> MSKLNAYFGEYGGQFVPQILVPALDQLEQEFIKAQADESFKQEFKELLQEYAGRPTALTKTRNIVKNTRTKLYLKREDLLHGGAHKTNQVLGQALLAKRMGKKEIIAETGAGQHGVATALACALLDLKCRVYMGAKDVERQSPNVFRMKLMGAEVIPVHSGSATLKDACNEALRDWSANYSKAHYLLGTAAGPHPFPTIVREFQRMIGEETKQQMLAKEGRLPDAVIACVGGGSNAIGMFADFIDEKNVKLIGVEPAGKGIETGEHGAPLKHGKTGIFFGMKAPLMQNSDGQIEESYSISAGLDFPSVGPQHAHLLAIGRAKYASAT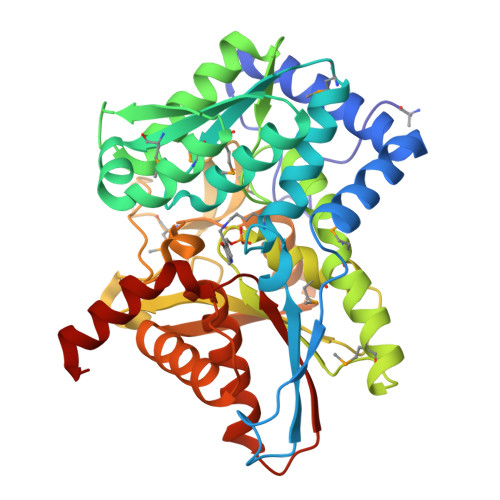DDEALDAFKLLCKKEGIIPALESSHALAHALKLAYEDPNKEQLLVVNLSGRGDKDIFTVHDILKEKGEI>[10x]MELYLDTSDVVAVKALSRIFPLAGVTTNPSIIAAGKKPLDVVLPQLHEAMG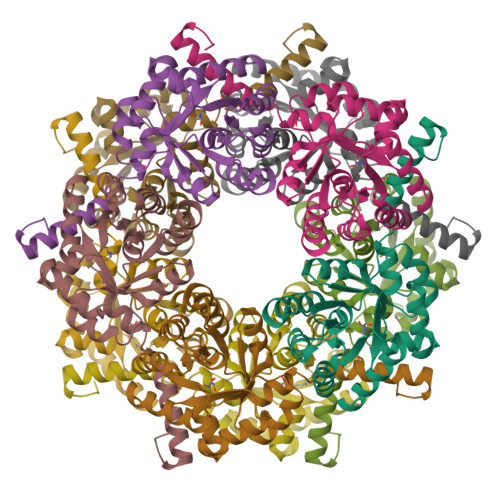GQGRLFAQVMATTAEGMVNDALKLRSIIADIVVKVPVTAEGLAAIKMLKAEGIPTLGTAVYGAAQGLLSALAGAEYVAPYVNRIDAQGGSGIQTVTDLHQLLKMHAPQAKVLAASFKTPRQALDCLLAGCESITLPLDVAQQMISYPAVDAAVAKFEQDWQGAFGRTSI> MKSSHHHHHHENLYFQSNAMENLGDKLSISQVYHLAQEYRDHAYSIANKIGSEEGLKQYYGLMNMSIQMFQLLKTKCTLSVLEDSKVTFEMVELLIQETYNFDLAELYISSLKERLQTHQSDTDLVEEIMRCEFLLLHDLPLMRDSKFHYKIALRNCNELVQYMVNLQDELYQNWASVFQYVGVMLCIKLKQHRRVKTSFHGLLSQCREKSQWKWFLNLCYVNYLLNERFPIPEDALQELRSTELHTVGPELYAWKLALEMVIQLCKDGNITDHLNEFKNFFDTNKQSLVTNEGKGCVIKIMPRIALKVELPMIFHYKELKNILLLLQSVSYIVNCYDEKGNFSRKFLPKVYSTTQKLIKNIAAGGVSMNELDSRIQTYKSILEFCEFYKVWEQTLLKGAVVTTESPKLGPSPGYVRLLQAMKVQFEGGGAVEEYTRLAQSGGTSSEVKMISLLNCYTVQAARVSRCSGDKQGELVEQCNKVWLQVEKLLQETDLQFNPIWECTVTILWLFSHFEPFSWNPLPCSDKQRAEYVSKLREFYSSNKFVAGEAVADNRFKLKKALLLQILVNYLGGRMLEHDLGEIYAISAKCFDMCRQQGGMRKVQYVIGIWHLMNCTVAMRGKDVALTNAKLEALVKQITSVKQ;> MKSSHHHHHHENLYFQSNAMSYPGKDKNIPGRIIEALEDLPLSYLVPKDGLAALVNAPMRVSLPFDKTIFTSAD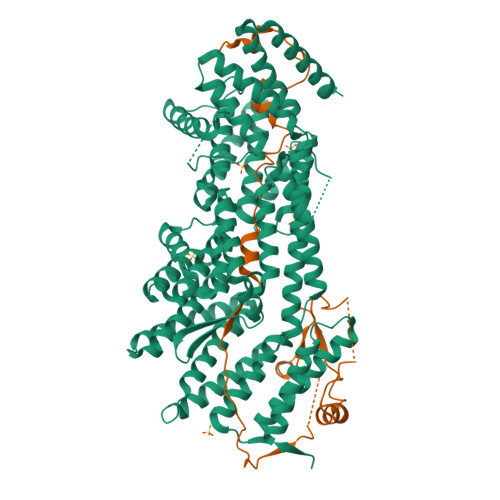DGRDVNINVLGTANSTTSSIKNEAEKERLVFKRPSNFTSSANSVDYVPTNFLEGLSPLAQSVLSTHKGLNDSINIEKKSEIVSRPEAKHKLESVTSNAGNLSFNDNSSNKKTKTSTGVTMTQANLA> MSQHNILEALNVRVVGTGDRILFLAHGFGTDQ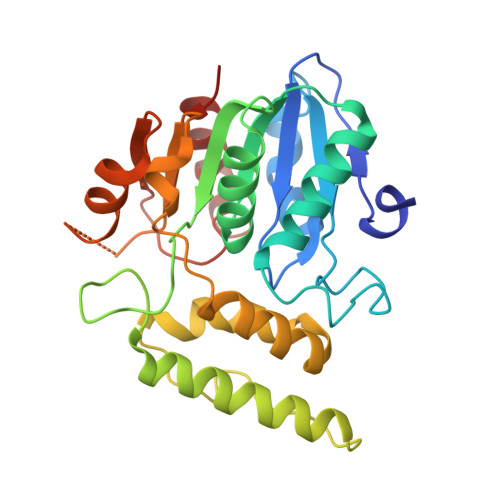SAWHLILPYFTQNYRVVLYDLVCAGSVNPDYFDFNRYTTLDPYVDDLLNIVDSLGIQNCAYVGHSVSAMIGIIASIRRPELFSKLILIGFSPRFLNDEDYHGGFEEGEIEKVFSAMEANYEAWVHGFAPLAVGADVPAAVREFSRTLFNMRPDISLFVSRTVFNSDLRGVLGLVRVPTCVIQTAKDVSVPASVAEYLRSHLGGDTTVETLKTEGHLPQLSAPAQLAQFLRRALPR> QDEISQDKWELARANNYLGLNLLKQLPSNDKTNVFFSPFSVSTAMGMAYAGARGDTLEQLTLNFGYAADELNEGKVLALFKEQLQSTNDLPHDYTLNIANAAVAQEGYGILPEYTDALTSSFGAEYIEADFQKRGQEAIQ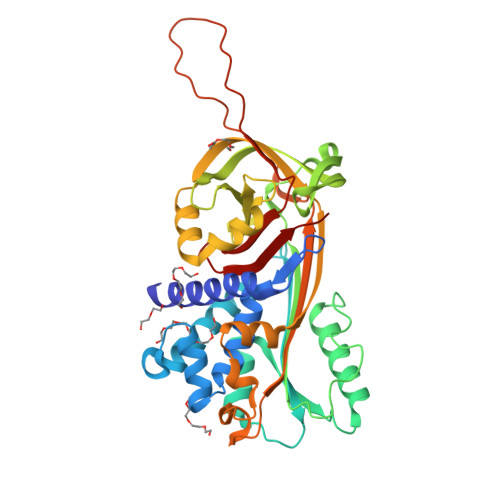KINAWVSNRTHGKVQSLFDEPPDFSTRLILLNAIYYKGTWLYEFDKTKTKPRSFYNGGVEKVQVPMMRLKSTLNHTYNAILNADLVDLPYVGNDFSMTIILPREKTGLASLKSVLTSQTLNLALQNMYPKDMKLKLPKFKLDTKYTLKPTLEAMGITKIFSADADLSGISGSRNLYVSDVLHKAVLEVNEEGSEAAAVTGFVIQLRTAAFVTPPPLPKVYVDHPFIFLIRNSKTNTIMFLGEINAL>MRIVQPVIEQLKAQSHPVCHYIYDLVGLEHHLQHITSSLPSNCQMYYAMKANSERTILDTISQYVEGFEVASQGEIAKGLAFKPANHIIFGGPGKTDEELRYAVSEGVQRIHVESMHELQRLNAILEDEDKTQHILLRVNLAGPFPNATLHMAGRPTQFGISEDEVDDVIEAALVMPNIHLDGFHFHSISNNLDSNLHVDVVKLYFKKAKSWSEKHRFPLKHINLGGGIGVNYADLTSQFEWDNFVENFKTLIVEQEMEDVTLNFECGRFIVAHIGYYVTEVLDIKKVHGAWYAILRGGTQQFRLPVSWQHNHPFEIYRYKDNPYSFEKVSISRQDTTLVGQLCTPKDVFAREVQIDAISTGDVIVFKYAGAYGWSIS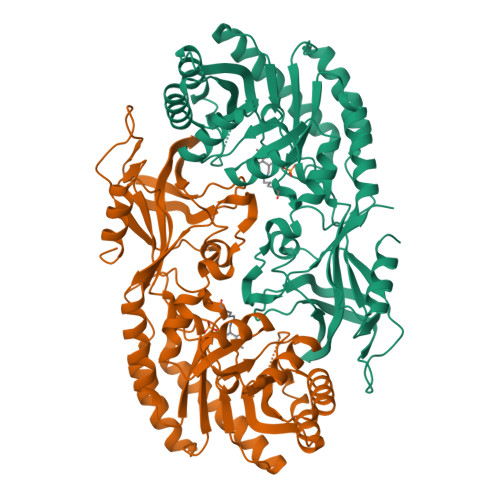HHDFLSHPHPEFIYLTQTKEDEHHHHHH[3x]>[2x]MFKGIV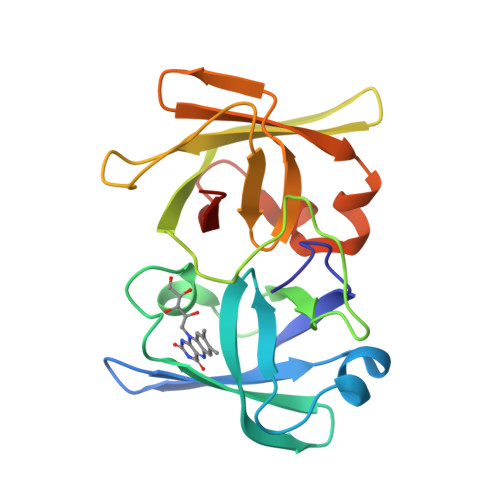QGAGIIKKISKNDDTQRHGITFPKDILESVEKGTVMLVNGCSLTVVRISGDVVYFDIDQAINTTTFRELEVGNKVNLEVRPEFGSLLGKGALTGNIKGVATVDNITEEEDRLKVYIKIPKDLIENILSEDHIGINGVSHSIEEISDDIIFINYPKNLSITTNLGTLEKGSDVNVETLNVSNEWD> MFFKEIHHVAINASNYQATKNFYVEKLGFEVLRENHRPEKN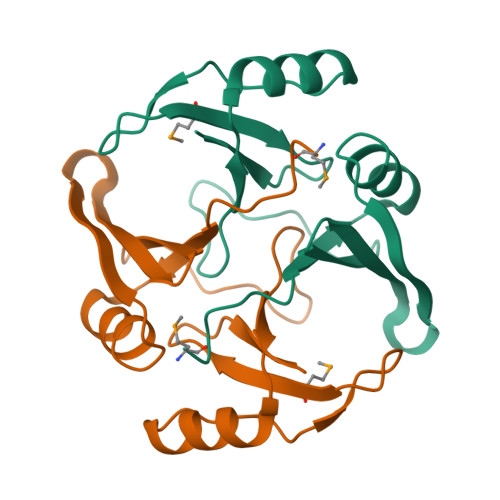DIKLDLKLGSQELEIFISDQFPARPSYPEALGLRHLAFKVEHIEEVIAFLNEQGIETEPLRVDDFTGKKMTFFFDPDGLPLELHE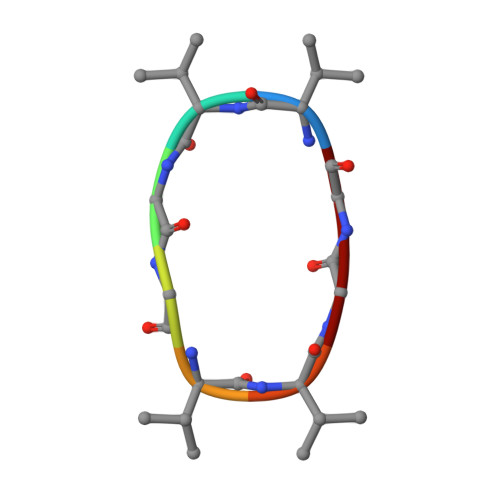> VVGGVVGG> GGAAGUGUACCUAGGGAUCCACCUCGAGAGAGGAAGGACCAAGCGGUACAGGCCUACUUCGGUAGGUUACA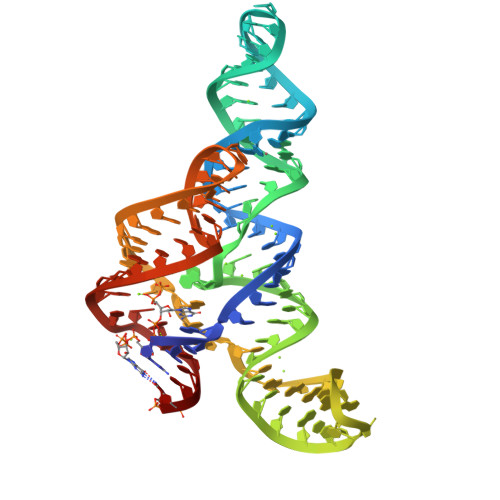CCGUGGGGAUAAAAGACCCGUGGCAAGUUUC>[4x]MAQERPSCAVEPEHVQRLLLSSREAKKSAYCPYSRFPVGAALLTGDGRIFSGCNIEN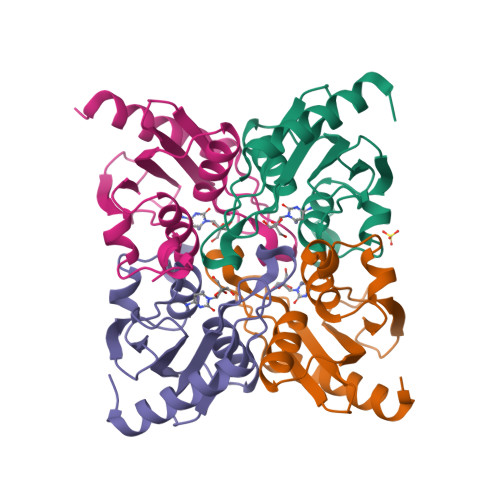ACYPLGVCAERTAIQKAISEGYKDFRAIAISSDLQEEFISPCGACRQVMREFGTDWAVYMTKPDGTFVVRTVQELLPASFGPEDLQKIQ>[2x]MQVNRLPFFTNHFFDTYLLISEDTPVGSSVTQLLARDMDNDPLVFGVSGE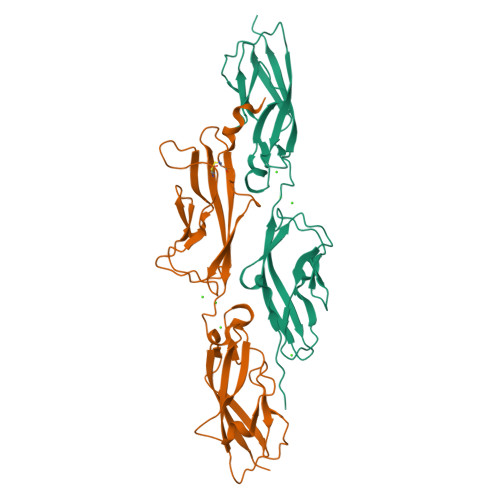EASRFFAVEPDTGVVWLRQPLDRETKSEFTVEFSVSDHQGVITRKVNIQVGDVNDNAPTFHNQPYSVRIPENTPVGTPIFIVNATDPDLGAGGSVLYSFQPPSPFFAIDSARGIVTVIQELDYEVTQAYQLTVNATDQDKTRPLSTLANLAIIITDLEHHHHHH;>[2x]MQYDDDWQYEDCKLARGGPPATIVAIDEESRNGTILVDNMLIKGTAGGPDPTIELSLKDNVDYWVLLDPVKQMLFLNSTGRVLDRDPPMNIHSIVVQVQCVNKKVGTVIYHEVRIVVRDRNDNSPTFKHESYYATVNELTPVGTTIFTGFSGDNGATDIDDGPNGQIEYVIQYNPEDPTSNDTFEIPLMLTGNVVLRKRLNYEDKTRYYVIIQANDRAQNLNERRTTTTTLTVDLEHHHHHH>MEEPEEPADSGQSLVPVYIYSPEYVSMCDSLAKIPKRAEMVHSLIEAYALHKQMRIVKPKVASMEEMATFHTDAYLQHLQKVSQEGDDDHPDSIEYGLGYDCPATEGIFDYAAAIGGATITAAQCLIDGMCKVAINWSGGWHHAKKDEASGFCYLNDAVLGILRLRRKFERILYVDLDLHHGDGVEDAFSFTSKVMTVSLHKFSPGFFPGTGDVSDVGLGKGRYYSVNVPIQDGIQDEKYYQICESVLKEVYQAFNPKAVVLQLGADTIAGDPMCSFNMTPVGIGKCLKYILQWQLATLILGGGGYNLANTARCWTYLTGVILGKTLSSEIPDHEFFTAYGPDYVLEITPSCRPDRNEPHRIQQILNYIKGNLKHVVIEG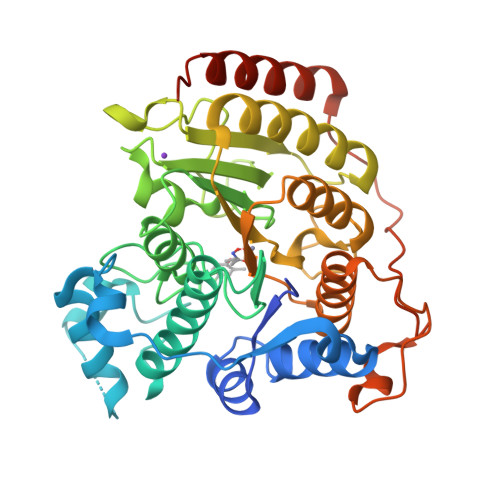RGSHHHHHH[2x]>[2x]MAEPAKVHGPKPTEESITKPRGPFEVNRRSVSRLKVKGFGGGTIYYPTNTTDGLFSAVSISPGFTGTQETMAWYGPRLASQGFVVFTIDTITTTDQPDSRARQLQASLKYLVNKSKVKDIIDPARLGVMGHSMGGGGSLKAALDNPKLKAAIPLTPWHTTKDFRGVRT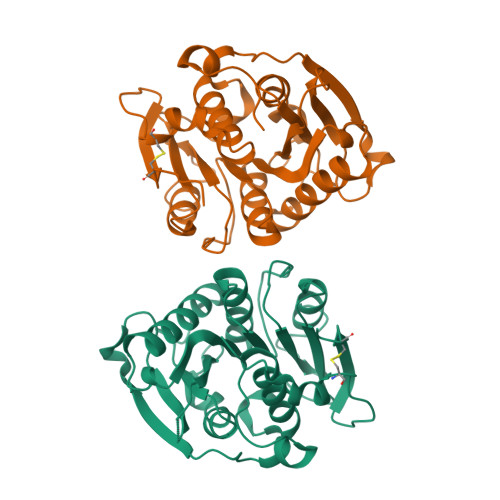PTLIIGAQNDTVAPVSQHAEPFYKSLPDKPGKAYLELAGASHLAPNTDNTTIAKFSIAWLKRFLDDDTRYDRFLCPPPRNNKSISDYRSTCPYKEHHHHHH> MRLSYEALEWRTPIENSTEPVSLPPPPPFFGQERAREALELAIRGGFHAYLVGPPSLGKHEALLAYLSTQSVETPPDLLYVPLSERKVAVLTLPSGQEIHLAEAVEGLLLEVNRLDELFRQGSFLREKTQLEARFKEAREQQLEALRREAQEAGFALSTNGERLELTGPGPVPAELSARLEEVTLGSLAASAELEVALRRLRRDWALHYLNNRFEPLFQRFPQARAYLEALRARLA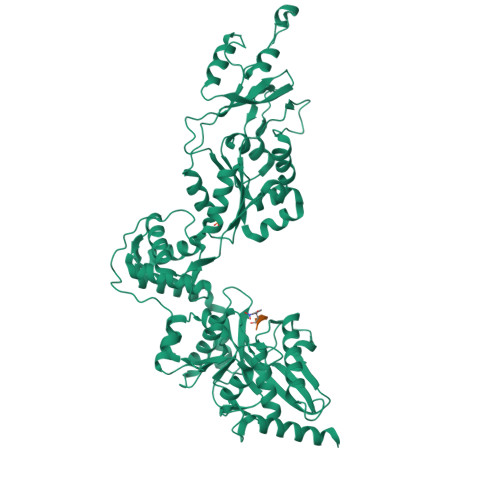RYAETGEPLDPAQWRPNLLTSSSSGTPPPIVYEPYATAPRLFGRLDYLVDRGVWSTNVSLIRPGAVHRAQGGYLILDALSLKREGTWEAFKRALRNGQVEPVTEPQAPAGLEVEPFPIQMQVILVGTPEAFEGLEEDPAFSELFRIRAEFSPTLPASPENCTALGGWLLAQGFQLTQGGLTRLYDEARRMAEQRDRMDARLVEIRALAEEAAVLGGGLLTAESVEQAIAAREHRSFLSEEEFLRAVQEGVIRLRTTGRAVGEVNSLVVVEAAPYWGRPARLTARAAPGRDHLISIDREAGLGGQIFHKAVLTLAGYLRSRYIEHGSLPVTISLAFEQNYVSIEGASAGLAELVAALSAIGNLPLRQDLAVTGAVDQTGKVLAVGAINAKVEGFFRVCKALGLSGTQGVILPEANLANLTLRAEVLEAVRAGQFHIYAVETAEQALEILAGARMEGFRGLQEKIRAGLEAFARLEEGHDKEDREKLAAALEHHHHHH;> EAVYA>[2x]GSMSFIPVAEDSDFPIQNLPYGVFSTQSNPKPRIGVAIGDQILDLSVIKHLFTGPALSKHQHVFDETTLNNFMGLGQAAWKEARASLQNLLSASQARLRDDKELRQRAFTSQASATMHLPATIGDYTDFYSSRQHATNVGIMFRGKENALLPNWLHLPVGYHGRASSIVVSGTPIRRPMGQMRPDNSKPPVYGACRLLDMELEMAFFV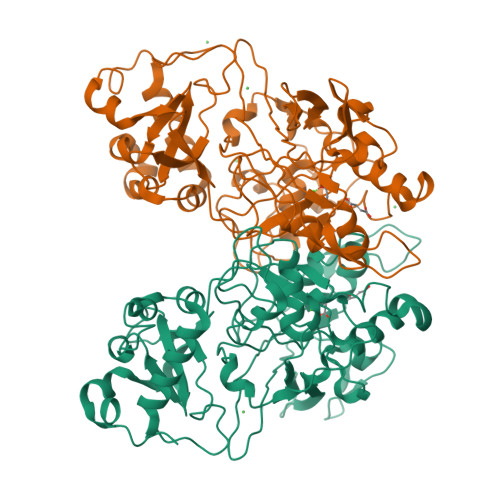GPGNRFGEPIPISKAHEHIFGMVLMNDWSARDIQQWEYVPLGPFLGKSFGTTISPWVVPMDALMPFVVPNPKQDPKPLPYLCHSQPYTFDINLSVSLKGEGMSQAATICRSNFKHMYWTMLQQLTHHSVNGCNLRPGDLLASGTISGSDPESFGSMLELSWKGTKAIDVGQGQTRTFLLDGDEVIITGHCQGDGYRVGFGQCAGKVLPALSPAGS> APAAPDKPLEFKGSQ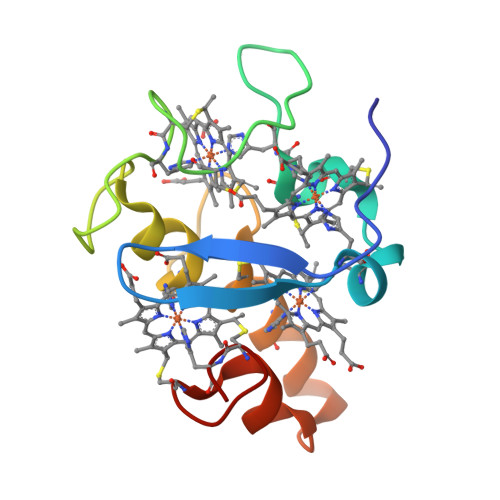KTVMFPHAVHAKVECVTCHHQVDGKESFAKCGSSGCHDDLAGKQGEKSLYYVVHTKKELKHTNCIGCHSKVVEGKPELKKDLTACAKSKCHP>MSVGTFSLPALPYAYDALEPSISAQIMELHHSKHHQTYVTNLNNALKTYSTALAANDVPSQIALQAAIKFNGAGHINHSLFWENLCPASSPDADPASAPELTAEIAKTWGSLDKFKEAMGKALLGIQGSGWGWLVKEGSGLRIVTTKDQDPVVGGEVPVFGIDMWEHAYYLQYLN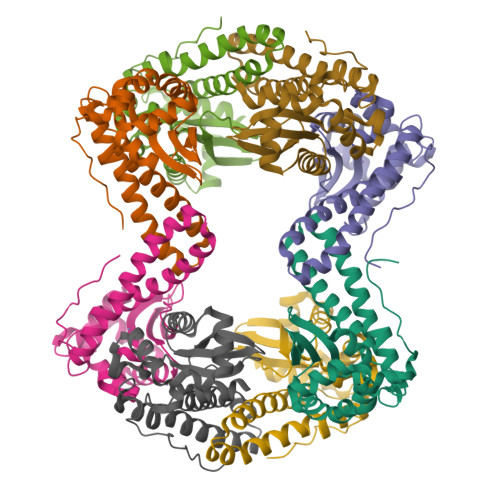GKAAYVDNIWKVINWKTAEQRFKGDREDAFKILKASL[8x]> GDYPLRVLYCGVCSLPTEYCEYMPDVAKCRQWLEKNFPNEFAKLT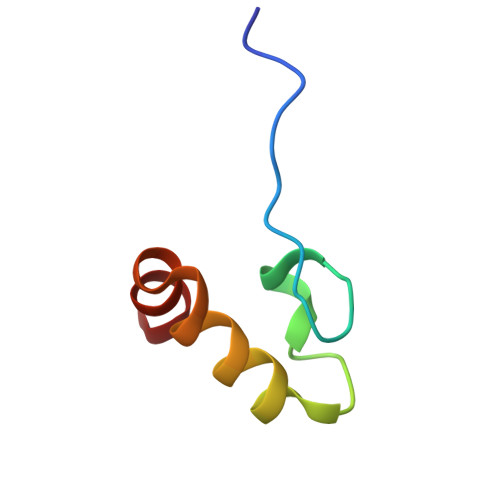V> MSFIKVGIKMGGLTSEQYHSQVVGKIGYIARCMQTIDPENNLKKIREDYQDVLIWAEKNYRFEEILEASKSGKCPNDLDALSRRSLILLELLRLVSSISPFKMKLDLIESQYEKMKQHVNLWKSDYHVKLNQLNQLTDYLKNAAPTPKNNFLRAMTSVLQMQIAQYGITEDNEGINQLFKLGLHLLAMANEKIDEQYHLFKGYVKDQPEESPFEGILPAEDQKILVKTMIDYAMPKLSSKVLQDKLSALSSSDVLTKTLLDSIDRIVKENEKLNALSKVKLGK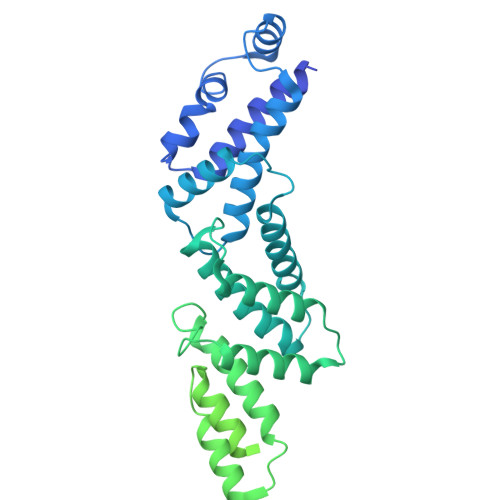FGLDIREIEVIYSQALKISPQDALQYTAQQCDAQLLSMAFPDSQNYIIESISNKKVKTIAELIHSKEFIYQIIKTEVFKQVDPNEKIRLQAATELYQLLGRIMDKQINLFTKMNLEQINEYIQTKTKAILDKIPERVELLTFMGFEIPTFKGIETLMTDISHSQDNETLAIAQEFYTNIKNAKNQLLGDKLIEDITPQDVEKFFNQCSQYGSEAAEKLADNRPVLTKIADILTAIARWAISLIGFNTPPQFLAPTRTCVDQVSDEITKIKLKLEDTLGSLQKVQEESLSL> MSSAHNAYNAGIMQKTGKAFADEFFAEENQVVHESNAVVLVLMKSDEIDAIIEDIVLKGGKAKNPSIVVEDKAGFWWIKADGAIEIDAAEAGELLGKPFSVYDLLINV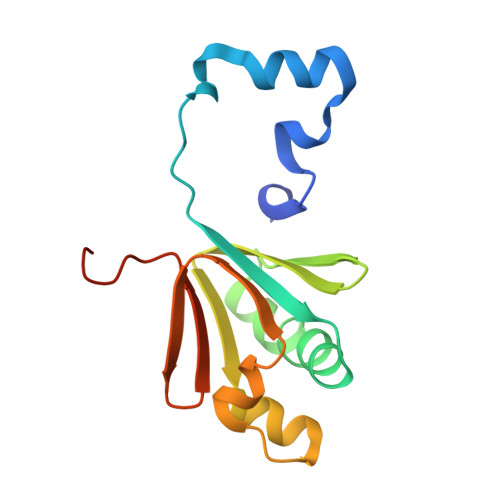SSTVGRAYTLGTKFTITSELMGLDRALTDI>[2x]MSKQSVTVIGLGPMGQAMVNTFLDNGHEVTVWNRTASKAEALVARGAVLAPTVEDALSANELIVLSLTDYDAVYAILEPVTGSLSGKVIANLSSDT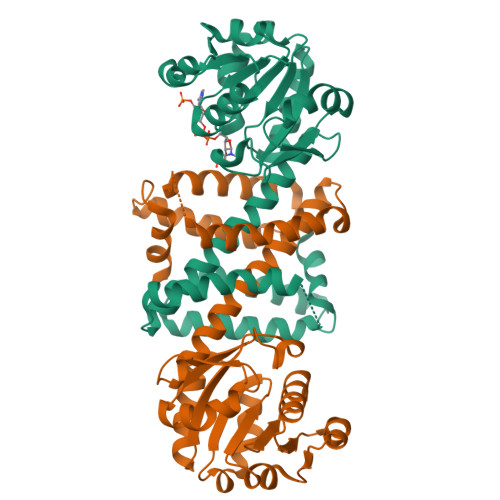PDKAREAAKWAAKHGAKHLTGGVQVPPPLIGKPESSTYYSGPKDVFDAHEDTLKVLTNADYRGEDAGLAAMYYQAQMTIFWTTMLSYYQTLALGQANGVSAKELLPYATMMTSMMPHFLELYAQHVDSADYPGDVDRLAMGAASVDHVLHTHQDAGVSTVLPAAVAEIFKAGMEKGFAENSFSSLIEVLKKPAV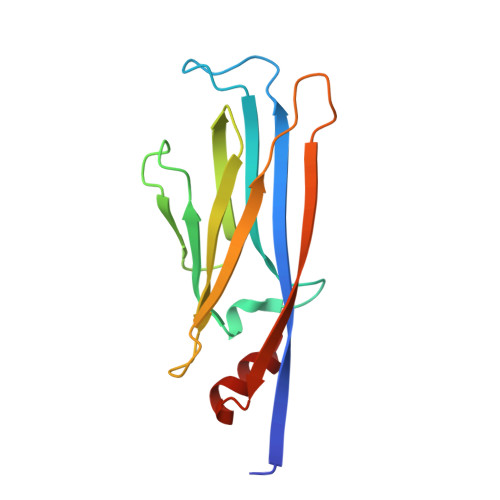> SHMASSCAVQVKLELGHRAQVRKKPTVEGFTHDWMVFVRGPEHSNIQHFVEKVVFHLHESFPRPKRVCKDPPYKVEESGYAGFILPIEVYFKNKEEPRKVRFDYDLFLHLEGHPPVNHLRCEKLTFNNPTEDFRRKLLKA> AGGHGDVGMHVKEKEKNKDENKRKDEERNKTQEEHLKEIMKHIVKIEVKGEEAVKKEAAEKLLEKVPSDVLEMYKAIGGKIYIVDGDITKHISLEALSEDKKKIKDIYGKDALLHEHYVYAKEGYEPVLVIQSSEDYVENTEKALNVYYEIGKILSRDILSKINQPYQKFLDVLNTIKNASDSDGQDLLFTNQLKEHPTDFSVEFLEQNSNEVQEVFAKAFAYYIEPQHRDVLQLYAPEAFNYMDKFNEQEINLSLEELKDQRMLSRYEKWEKIKQHYQHWSDSLSEEGRGLLKKLQIPIEPKKDDIIHSLSQEEKELLKRIQIDSSDFLSTEEKEFLKKLQIDIRDSLSEEEK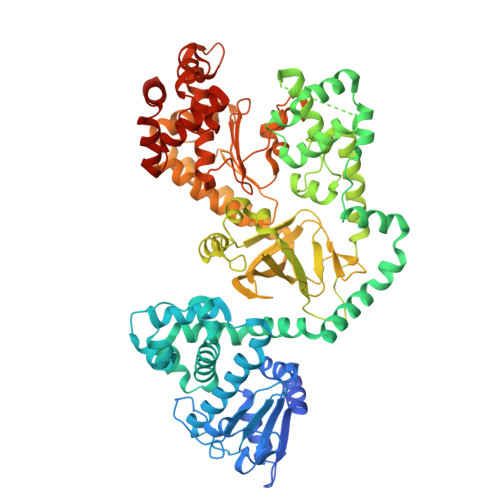ELLNRIQVDSSNPLSEKEKEFLKKLKLDIQPYDINQRLQDTGGLIDSPSINLDVRKQYKRDIQNIDALLHQSIGSTLYNKIYLYENMNINNLTATLGADLVDSTDNTKINRGIFNEFKKNFKYSISSNYMIVDINERPALDNERLKWRIQLSPDTRAGYLENGKLILQRNIGLEIKDVQIIKQSEKEYIRIDAKVVPKSKIDTKIQEAQLNINQEWNKALGLPKYTKLITFNVHNRYASNIVESAYLILNEWKNNIQSDLIKKVTNYLVDGNGRFVFTDITLPNIAEQYTHQDEIYEQVHSKGLYVPESRSILLHGPSKGVELRNDSEGFIHCFGHAVDDYAGYLLDKNQSDLVTNSKKFIDIFKEEGSNLTSYGRTNEAEFFAEAFRLMHSTDHAERLKVQKNAPKTFQFINDQIKFIINS> QAEWRSWEVNKRLEYSLVKGITEFIEQDTEEARQQATRPIEVIEGPLMDGMNVVGDLFGEGKMFLPQVVKSARVMKQAVAYLEPFIEASKEQGKTNGKMVIATVKGDVGDIGKNIVGVVLQCNNYEIVDLGVMVPAEKILRTAKEVNADLIGLSGLITPSLDEMVNVAKEMERQGFTIPLLIGGATTSKAHTAVKIEQNYSGPTVYVQN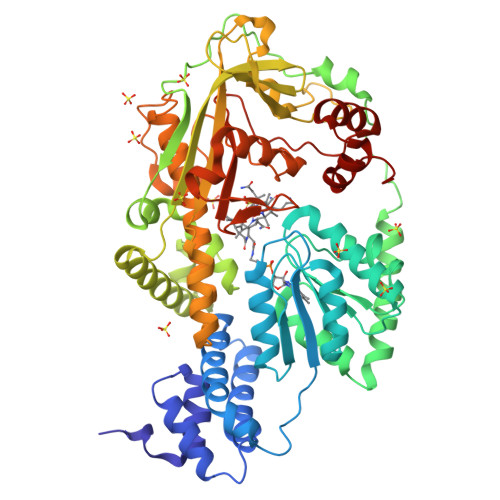ASRTVGVVAALLSDTQRDDFVARTRKEYETVRIQHGRKKPRTPPVTLEAARDNDFAFDWQAYTPPVAHRLGVQEVEASIETLRNYIDWTPFFMTWSLAGKYPRILEDEVVGVEAQRLFKDANDMLDKLSAEKTLNPRGVVGLFPANRVGDDIEIYRDETRTHVINVSHHLRQQTEKTGFANYCLADFVAPKLSGKADYIGAFAVTGGLEEDALADAFEAQHDDYNKIMVKALADRLAEAFAEYLHERVRKVYWGYAPNENLSNEELIRENYQGIRPAPGYPACPEHTEKATIWELLEVEKHTGMKLTESFAMWPGASVSGWYFSHPDSKYYAVAQIQRDQVEDYARRKGMSVTEVERWLAPNLGYDAD>[3x]GSVDQNIPRGAVLHSEPLTVMVLTATDPFEYESPEHEVKNMLHATVATVSQYFHVKVFNINLKEKFTKKNFIIISNYFESKGILEINETSSVLEAAPDQMIEVPNSIIRNANASPKICDIQKGTSGAVFYGVFTLHKKTVNRKNTIYEIKDGSGSI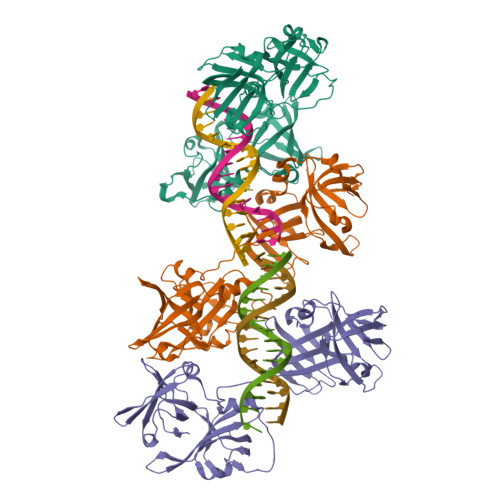EVVGSGKWHNINCKEGDKLHLFCFHLKTIDRQPKLVCGEHSFIKISKRGNVPKEPAKEEDHHHGPKQVMVLKVTEPFTYDLKEDKRMFHATVATETEFFRVKVFDTALKSKFIPRNIIAISDYFGCNGFLEIYRASCVSDVNVNPTMVISNTLRQRANATPKISYLFSQARGTFVSGEYLVNKKTERNKFIYYGIGDDTGKMEVVVYGRLTNVRCEPGSKLRLVCFELTSTEDGWQLRSVRHSYMQVINARKAAAS>MGDNIVLYYFDARGKAELIRLIFAYLGIEYTDKRFGVNGDAFVEFKNFKKEKDTPFEQVPILQIGDLILAQSQAIVRYLSKKYNICGESELNEFYADMIFCGVQDIHYKFNNTAANETTFLNEDLPKWSGYFEKLLKKNHTNNNNDKYYFVGNNLTYADLAVFNLYDDIETKYPSSLKNFPLLKAHNEFI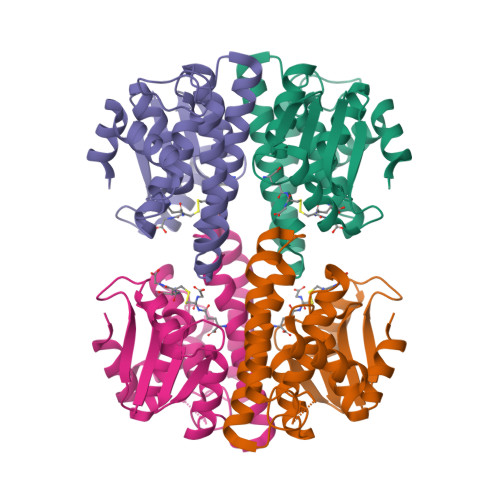SNLPNIKNYITNRKESVY[2x]>GHMPNPVRFVYRVDLRSPEEIFEHGFSTLGDVRNFFEHILSTNFGRSYFISTSETPTAAIRFFGSWLREYVPEHPRRAYLYEIRADQHFYNARATGENLLDLMRQRQVVFDSGDREMAQMGIRALRTSFAYQREWFTDGPIAAANVRSAWLVDAVPVEPGHAHHPAGRVVETTRINEPEMHNPHYQELQTQANDQPWLPTPGIATPVHLSIPQAASVADVSEGTSASLSFACPDWSPPSSNGENPLDKCIAEKIDNYNLQSLPQYASSVKELEDTPVYLRGIKTQKTFMLQADPQNNNVFLVEVNPKSSFPQTIFFWDVYQRICLKDLTGAQISLSLTAFTTQYAGQLKVHLSVSAVNAVNQKWKMTPQDIAITQFRVSSELLGQTENGLFWNTKSGGSQHDLYVCPLKNPPSDLEELQIIVDECTTHAQFVTMRAASTFFVDVQLGWYWRGYYYTPQLSGWSYQMKTPDGQIFYDLKTSKIFFVQDNQNVFFLHNKLNKQTGYSWDWVEWLKHDMNEDK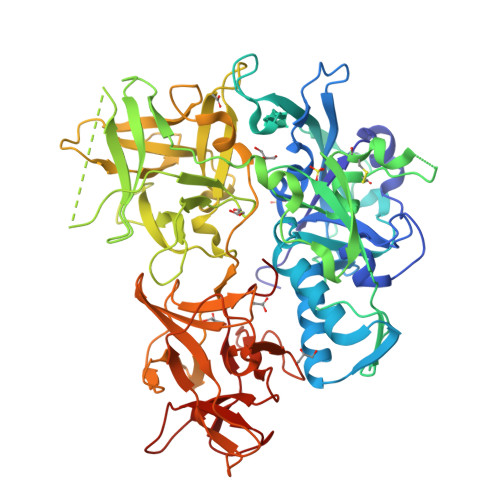DENFKWYFSRDDLTIPSVEGLNFRHIRCYADNQQLKVIISGSRWGGWYSTYDKVESNVEDKILVKDGFDRF[6x]Herein, we demonstrate the inhibitory activity of taniborbactam against PenI, the class A β-lactamase produced by B. pseudomallei. PenI was found to be an extended-spectrum β-lactamase (ESBL). Taniborbactam is a boronic acid β-lactamase inhibitor with a broad spectrum of activity that covers not only class A, C, and D serine β-lactamases but also many class B metallo-β-lactamases, including NDM (except NDM-9 and NDM-30) and VIM (except VIM-83). In conclusion, we demonstrated that PenI, the main mechanism of resistance to β-lactams in the pathogen B. pseudomallei, is effectively overcome by potent inhibition by taniborbactam.

The PenI–taniborbactam complex structure was solved in space group P21 at 1.25 Å resolution. The tail end of taniborbactam could not be resolved, as poor electron density was observed for the 2Fo-Fc map at 1.0 σ and the polder map (omit map) at 2.5 σ in this region; thus, the atom occupancies were set to 0.3. The high resolution of the active site allowed detection of the boron of taniborbactam bound to Ser70, as well as other direct hydrogen-bonding interactions of taniborbactam with residues Ser130, Asn132, Thr235, and Thr237 and water-bridged hydrogen-bonding interactions with Glu166 and Thr216. Therefore, the overall binding mode was like that observed in the KPC-2 structure in complex with taniborbactam, with some differences. For instance, the orientation of Tyr105 in PenI was different from that of Trp105 in the KPC-2/taniborbactam complex. In PenI, Tyr105 limited the freedom of taniborbactam to have alternate conformations. Also, in the PenI–taniborbactam complex, a disulfide bond between Cys77 and Cys123 as well as free thiols was observed with the ratio between the two at approximately 1:1. Of note, in the apo-PenI structure, only the free thiols were observed; thus, a disulfide bond appears to have formed upon complexing with taniborbactam. As the disulfide bond was not observed in the apo-PenI structure, we hypothesize that the binding of taniborbactam induces a conformational change that slightly shortens the distance between the Cys residues, allowing the formation of the disulfide bond. Thus, it is likely that the binding of taniborbactam by PenI led to the formation of the disulfide bond between Cys77 and Cys123, which would increase the stability of the PenI–taniborbactam complex and the residence time for the presence of taniborbactam in the complex.

> NVAAAERQLRELESTFDGRLGFVALDTATGARIAHRGDERFPFCSTSKMMLCAAVLARSAGEPALLQRRIAYAKGDLIRYSPITEQHVGAGMSVAELCAATLQYSDNTAANLLIALLGGPQTVTAYARSIGDATFRLDRREPELNTALPGDERDTTTPAAMAASVHRLLVGDALGAAQRAQLNAWMLGNKTGDARIRAGVPADWRVADKTGTGDYGTANDIGVAYPPNRAPIVFIVYTTMRNPNAQARDDVIASATRIAARAFA>PKHGKRYRALLEKVDPNKIYTIDEAAHLVKELATAKFDETVEVHAKLGIDPRRSDQNVRGTVSLPHGLGKQVRVLAIAKGEKIKEAEEAGADYVGGEEIIQKILDGWMDFDAVVATPDVMGAVGSKLGRILGPRGLLPNPKAGTVG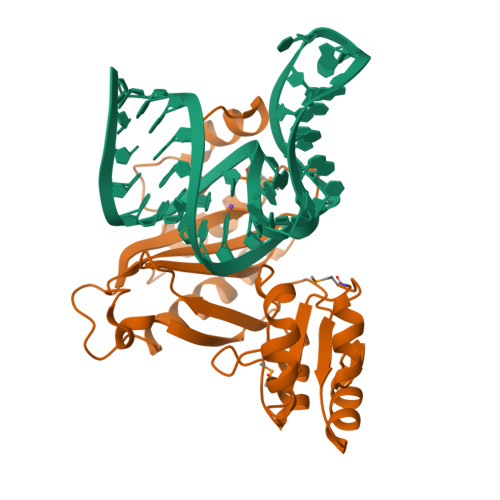FNIGEIIREIKAGRIEFRNDKTGAIHAPVGKASFPPEKLADNIRAFIRALEAHKPEGAKGTFLRSVYVTTTMGPSVRINPHS[4x]>GSMDQPAGLQVDYVFRGVEHAVRVMVSGQVLELEVEDRMTADQWRGEFDAGFIEDLTHKTGNFKQFNIFCHMLESALTQSSESVTLDLLTYTDLESLRNRKMGGRPGSLAPRSAQLNSKRYLILIYSVEFDRIHYPLPLPYQGKP[3x]

The highly conserved coiled-coil domain-containing protein 61 (CCDC61, also known as variable flagellar number 3, VFL3) is one of these understudied proteins. Here, we identify CCDC61 as a highly conserved paralog of SAS6, a key organizer of the central scaffold around which centrioles are formed (Leidel et al., 2005). Our crystal structures of CCDC61 demonstrate that it adopts a SAS6-like fold and forms oligomers through two homodimerization domains in a similar way to SAS6: an N-terminal globular head and a parallel coiled-coil domain. Further analysis of CCDC61 reveals that its coiled-coil domains are capable of directly interacting with microtubules.

To gain more insight into the domain organization of CCDC61, we determined the crystal structure of the N-terminal domain of human CCDC61 (hCCDC611−143) at a resolution of 2.6 Å using X-ray crystallography. As indicated by our bioinformatics analyses, we found that the protein fold of CCDC61 is remarkably similar to the canonical SAS6/XRCC4-like fold, which is characterized by the presence of a seven-stranded β barrel with a helix-turn-helix motif inserted between β4 and 5. CCDC61 has an insertion of an extra α helix (α3) followed by an unstructured loop between β5 and β6, which are unique to CCDC61. The asymmetric unit of the hCCDC611−143 crystal contained three copies of protomers that pack tightly against each other through interface regions whose residues are evolutionary conserved (D1 and D2). Remarkably, one observed CCDC61 homodimer (D1) is highly similar to that formed by the SAS6 head domain (van Breugel et al., 2011, Kitagawa et al., 2011). The conserved phenylalanine F128 of hCCDC61 (asterisks in Figures 2A, close up in (i) and S1B, dark blue arrow in the alignment) makes van der Waals interactions with M70 and V82 lining a hydrophobic pocket of the homodimer partner that is constituted by α2, the β hairpin of β5 and 6, and the turns before and after α2 (Figure 2A, in (i)). The dimer interface is further stabilized by an extensive network of salt bridges and hydrogen bonds, including a β zipper formed by residues found between α1 and α2. To test whether homodimer formation of hCCDC611−143 observed in crystallo is also observed in solution, we studied the oligomeric state of the protein using analytical ultracentrifugation (AUC). This analysis suggests that hCCDC611−143 exists in a monomer-dimer equilibrium with a KD of 170 ± 18 μM, suggesting a relatively weak binding affinity, similar to that observed with SAS6 (van Breugel et al., 2011, Kitagawa et al., 2011). Thus, the overarching principles of higher-order oligomerization and stabilization by other proteins appears to be conserved among the XRCC4 superfamily members. It is worth mentioning that the head domain of hCCDC61 contains a conserved surface area that is not directly involved in D1 dimer formation as described in Figures 2A and S2A.>[2x]MKKILAINFSTASKKGEGTGYAFRKDGQVYVGSIKAYNPKKTAWERTFDIVNA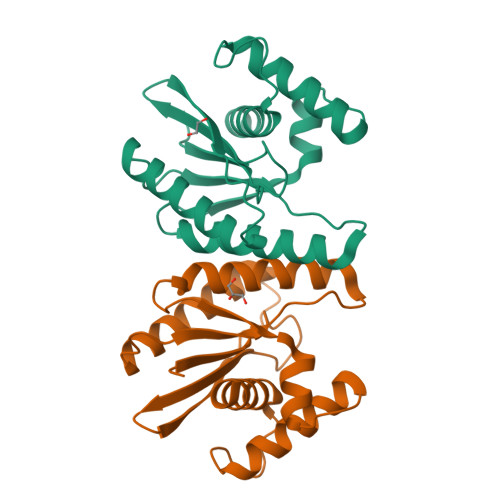IKDIIDEFDLKGYHLAIETPIMGRNRKHSITLANCNGYFIGAIDGLVNGYTFIDNSKWCSYHLISGKREQRKEESLELLKATGLVDSNCKDDNIADAYNILTYCEHLG> MATDKEAKDVIDKFIDNVFNFDVLTKERIKEKDEEIKKITTDDMYEKVVYIRPYVGVIQSLNPQHVQYESFSNNGYDIEAELSFRKVSYLVDKGSIPTDSLSTLTVHLVERNQELLIDYFDEIQDVLYGEYMEEEYVFDEDVPLSTILALDLNDNLKSLSNIKYMFKGAPKENPFGTDKDVYIDTYNLLYWLYLGEDEELAYPMNINYFFTEGRFFTIFGKGHKYKVDVSKFIVGDILFFGRSDTNIGIYVGDGEFISMMGKFPKDETPIGKYKLDDYWNEFNGRVMRFDEEVYI;> MVVRFQSSMGRSLKRVDSDDLNVKGLVLATVSKINYKYQSVEVKVNNLTLGSRIGDDGSLAVPYPKSFIGRTPEGSVFGTKPLITEGSVVLIGFLNDDINSPIILSVYGDNEQNKMINTNPLDGGKFDTESVYKYSSSLYEILPSLNYKYDDGEGTSIRTYNGKSFFSMTSGEEEKPQATDFYTGTEYQDLFTSYYGNKTLIEPRIQKAPNMLFKHQGVFYDDGTPDNHITTLFISERGDIRASVLNTETQKRTTQEMSSDGSYRVIKQDDDLMLDEAQVWIEYGISEDNKFYIKNDKHKFEFTDEGIYIDDKPMLENLDESIAEAMKNLNEIQKELDDINYLLKGVGKDNLEELIESTKESIEASKKATSDVNRLTTQIAEVSGRTEGIITQFQKFRDETFKDFYEDASTVINEVNQNFPTMKTDVKTLKTKVDNLEKTEIPNIKTRLTELENNNNNADKIISDRGEHIGAMIQLEENVTVPMRKYMPIPWSKVTYNNAEFWDSNNPTRLVVPKGITKVRVAGNVLWDSNATGQRMLRILKNGTYSIGLPYTRDVAISTAPQNGTSGVIPVKEGDYFEFEAFQDSEGDRQFRADPYTWFSIEAIELETETMEKDFMLIGHRGATGYTDEHTIKGYQMALDKGADYIELDLQLTKDNKLLCMHDSTIDRTTTGTGKVGDMTLSYIQTNFTSLNGEPIPSLDDVLNHFGTKVKYYIETKRPFDANMDRELLTQLKAKGLIGIGSERFQVIIQSFARESLINIHNQFSNIPLAYLTSTFSESEMDDCLSYGFYAIAPKYTTITKELVDLAHSKGLKVHAWTVNTKEEMQSLIQMGVDGFFTNYLDEYKKI;>MKTRKLTNILSKLIDKTMAGTSKITDFTPGSASRSLLEAVSLEIEQFYILTKENIDWGIQEGIIEAFDFQKRQSKRAYGDVTIQFYQPLDMRMYIPAGTTFTSTRQEYPQQFETLVDYYAEPDSTEIVVEVYCKETGVAGNVPEGTINTIASGSSLIRSVNNEYSFNTGTKEESQEDFKRRFHSFVESRGRATNKSVRYGALQIPDVEGVYVYEETGHITVFAHDRNGNLSDTLKEDIIDALQDYRPSGIMLDVTGVEKEEVNVSATVTISNKSRIGDTLQKHIESVIRSYLNNLKTSDDLIITDLIQAIMNIDDVLIYDVSFDNLDENIIVPPQGIIRAGEIKVELK[4x];> MRRIRRPKVRIEIVTDDNTFTLRFEDTRDYNGDEFGAKLLGFQTKNSMEDDSSVFQINMAGDTYWDKLVMANDIIRIFITPNDDPNDKEGKQERLIQVGMVSQVSKVGSYGNDQTQFRITGQSFVKPFMKFGLGVIQEVQAVLPEVGWLIDGDGDNEVKFTGSSAHEVMTGIIRRFIPYMKYNYTEKTYNTIDNYLDYDDLSSWDEFEKLTEVSAFTNFDGSLKQLMDMVTARPFNELFFKNSEKTPGKAQLVLRKTPFNPTEWRALDMIKVPTEDFIEEDVGKSDVETYSIFTATPAGMLKELNGDVFSKPQFHPELTDRYGYTKFEVENIYLSTKSGSATEDSDSSGDDNGTERGTYSKIMKDLSNYGRDNISKGIDKYTSKLSSKYKNLKKAQAKKIIEKFVKEGKVTEKEYEKITGNKVDDELTSDNRPKLTKDKLKSILKEKFKTQDDFNNSKKKKKAKTDALKELTTKYRFGNKTHATTLLDEYIKYKGEPPNDEAFDKYLKAIEGVSNVATDTGSDASDSPLVMFSRMLFNWYHGNPNFYAGDIIVLGDPKYDLGKRLFIEDKQRGDTWEFYIESVEHKFDYKQGYYTTVGVTRGLKDAILEDGKGSPHRFAGLWNQSSDFMGGLMGEDTSKELKEKGVAEKQSSGDKDGGSDSGGAQDGGSLDSLKKYNGKLPKHDPSFVQPGNRHYKYQCTWYAYNRRGQLGIPVPLWGDAADWIGGAKGAGYGVGRTPKQGACVIWQRGVQGGSPQYGHVAFVEKVLDGGKKIFISEHNYATPNGYGTRTIDMSSAIGKNAQFIYDKK;>MNNFIPQPQGLLRFLNTLDTDLTSSHMNLLDEEVSFVSKFYTPQLQLSELAKKVLTNIKTDDIPVLEREFNDNTIIHKANDTLLKVQAPRMYMILQSIVLEAYAIVNCFVENPSSLKYLTEEDVSITRENLNYVADYLGNYDDYNSVVLDLRDLDLCFSAIELQLPLIKKEANV[2x];>[2x]MANFLKNLHPLLRRDRNKKDNQDPNFALIDALNEEMNQVEKDAIESKLQSSLKTSTSEYLDKFGDWFGVYRKTDEKDDVYRARIIKYLLLKRGTNNAIIDAIKDYLGRDDIDVSVYEPFTNIFYTNKSHLNGEDHLMGYYYRFAVINVSIGDYFPVEIIDVINEFKPAGVTLYVTYDGASTIRGGAIIKWLDGLPKIETYQEFDRFTGYDDTFYGHINMNQSKDTDNSSSDIFKTNHSLINSLDVLTGSSSVGRQYINYGYVTSYVYNPGMTSSVNQISASTEGRGQEVPTDYYMYTSTKNNNTVELSMQTTSGVSYLYNNFNFRDYMSKYRPQVDLQSDEARRIVSDYIKELSIDYYLSAVIPPDESIEIKLQVYDFSINRWLTVSINNLSFYEKNIGSNIGYIKDYLNSELNMFTRLEINAGKRDSVDIKVNYLDLMFYYYERGIYTIKPYKALIENYLDISRETYVEAFKIASLSNGDIITKTGFQPIGYLKLVGNYENTIPSTINIVAKDTDNNPIESNELDVYNTVENRNLLQSYKGVNTIAREITS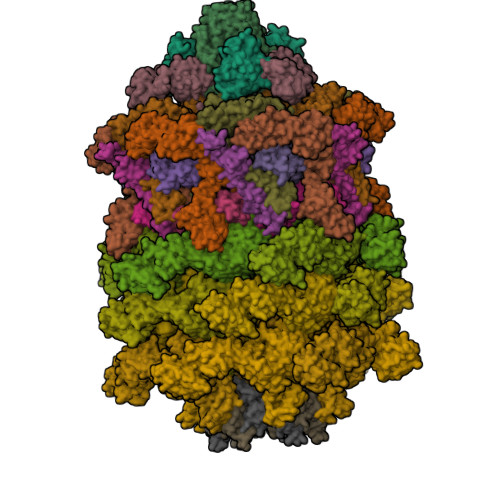TKEFTVSGWAKEIYSTNYLSKVLKPGKVYTLSFDMEITGNDPTLKSYSDNHGIYLYSNTKGIVVNGVKSMERTIGNKVSVTQTFTAPTITDHRLLIYTGRYTSDGKASTPPVFFNTVKITELKLTEGSSKLEYSPAPEDKPNVIEKGIKFNNILTNIQTLSINSDTILKNVTLYYSYYGDSWVELKTLGNISTGETTETNNLIDLYGLQTVDYSNINPMSKVSLRSIWNVKLGELNNQEGSLSNMPNDYFNAVWQDIDKLSDIELGSMRMVKDTEGGVFDGATGEIIKATLFNVGAYTDLDMLAYTLTNYTEPLTLGSSRLISELKEELLTSESFNVDNRIKVIDSIYEELPNTSIIKNGFVEREVTGSKYLDYGLYEPIEDGTRYKLIVEGEFKDNIEFISLYNSNPNFNETFIYPSEIINGVAEKEFIAKPSTEDKPRLNTDVRIYIRPYDSTISKVRRVELRKV;>MRFKKHVVQHEETMQAIAQRYYGDVSYWIDLVEHNNLKYPYLVETDEEKMKDPERLASTGDTLIIPIESDLTDVSAKEINSRDKDVLVELALGRDLNITADEKYFNEHGTSDNILAFSTNGNGDLDTVKGIDNMKQQLQARLLTPRGSLMLHPNYGSDLHNLFGLNIPEQATLIEMEVLRTLTSDNRVKSANLIDWKIQGNVYSGQFSVEIKSVEESINFVLGQDEEGIFALFE[2x];>MPQSDGISNLHRIALRFPKEGGGYDMYRFKVNPENYTIDSPQRTTAIKTKSDIVIEDYGKDIEVINFTGTTGFRPVREADGLKTGKQKMEELQSRVSEYAMQGGSGNVSGSYLQFFNFTDDSYYKVHLAPQGLKITRSKDEPLLFRYEITLVVIGSLTEADRSAVTTEEFGNVKPNASQRVDEGIKELDKNARKTRDRNNQEISRRENTIPKSTGDNTNEGNRLKQSFPSSSIYNPRQSTNGLKGNIDNMALIIGYGDGGVSS[2x];>[6x]MAVEPFPRRPITRPHASIEVDTSGIGGSAGSSEKVFCLIGQAEGGEPNTVYELRNYSQAKRLFRSGELLDAIELAWGSNPNYTAGRILAMRIEDAKPASAEIGGLKITSKIYGNVANNIQVGLEKNTLSDSLRLRVIFQDDRFNEVYDNIGNIFTIKYKGEEANATFSVEHDEETQKASRLVLKVGDQEVKSYDLTGGAYDYTNAIITDINQLPDFEAKLSPFGDKNLESSKLDKIENANIKDKAVYVKAVFGDLEKQTAYNGIVSFEQLNAEGEVPSNVEVEAGEESATVTATSPIKTIEPFELTKLKGGTNGEPPATWADKLDKFAHEGGYYIVPLSSKQSVHAEVASFVKERSDAGEPMRAIVGGGFNESKEQLFGRQASLSNPRVSLVANSGTFVMDDGRKNHVPAYMVAVALGGLASGLEIGESITFKPLRVSSLDQIYESIDLDELNENGIISIEFVRNRTNTFFRIVDDVTTFNDKSDPVKAEMAVGEANDFLVSELKVQLEDQFIGTRTINTSASIIKDFIQSYLGRKKRDNEIQDFPAEDVQVIVEGNEARISMTVYPIRSFKKISVSLVYKQQTLQA;>MASEAKQTVHTGNTVLLMIKGKPVGRAQSASGQREYGTTGVYEIGSIMPQEHVYLRYEGTITVERLRMKKENFADLGYASLGEEILKKDIIDILVVDNLTKQVIISYHGCSANNYNETWQTNEIVTEEIEFSYLTASDKART[6x]>GSMSLIIC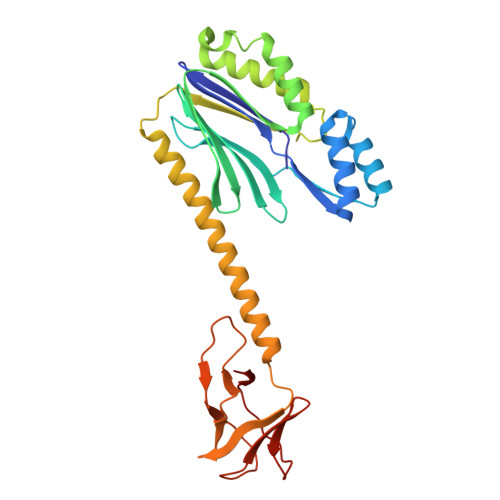YYGKNGAVIGGDRRQIFFRGSEENRKILEEKLYSGEIKSEEELYKLAEKLNIKIIIEDDREKVRKISDSVVCGEVRSLGIDAKRRRVYATKGKCAIVDILNDTVTNQTIKEGFGIVVLGNRFLKKKAEEELKRTAKLFPMMPIQQIEDAIKEIFEKLKWHPTVSKEYDIYSVNKYEKNFEEVIKKDIESLFKYREQLRKQLIDFGKVMSIVNKIVKNGEIGVIKDGKLHLYDDYIAIDKIDPNPKVFKVVDVEGNFKDGDIVVIENGDMKIKGTNEKVTTKYIIIHK[4x]>MSAKSRTIGIIGAP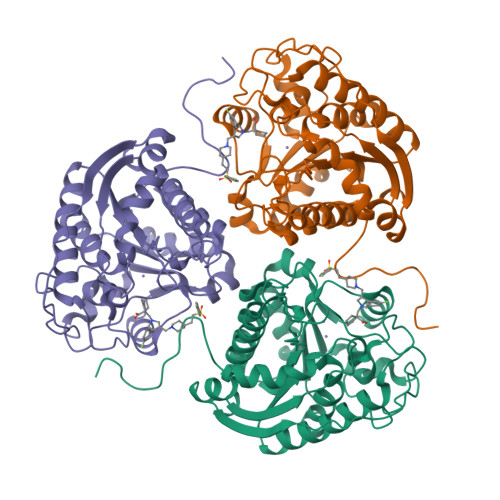FSKGQPRGGVEEGPTVLRKAGLLEKLKEQECDVKDYGDLPFADIPNDSPFQIVKNPRSVGKASEQLAGKVAEVKKNGRISLVLGGDHSLAIGSISGHARVHPDLGVIWVDAHTDINTPLTTTSGNLHGQPVSFLLKELKGKIPDVPGFSWVTPCISAKDIVYIGLRDVDPGEHYILKTLGIKYFSMTEVDRLGIGKVMEETLSYLLGRKKRPIHLSFDVDGLDPSFTPATGTPVVGGLTYREGLYITEEIYKTGLLSGLDIMEVNPSLGKTPEEVTRTVNTAVAITLACFGLAREGNHKPIDYLNPPK[6x]> STAKAPTLPASIFRAYDIRGVVGDTLTAETAYWIGRAIGSESLARGEPCVAVGRDGRLSGPELVKQLIQGLVDCGCQVSDVGMVPTPVLYYAANVLEGKSGVMLTGSHNPPDYNGFKIVVAGETLANEQIQALRERIEKNDLASGVGSVEQVDILPRYFKQIRDDIAMAKPMKVVVDCGNGVAGVIAPQLIEALGCSVIPLYCEVDGNFPNHHPDPGKPENLKDLIAKVKAENADLGLAFDGDGDRVGVVTNTGTIIYPDRLLMLFAKDVVSRNPGADIIFDVKCTRRLIALISGYGGRPVMWKTGHSLIKKKMKETGALLA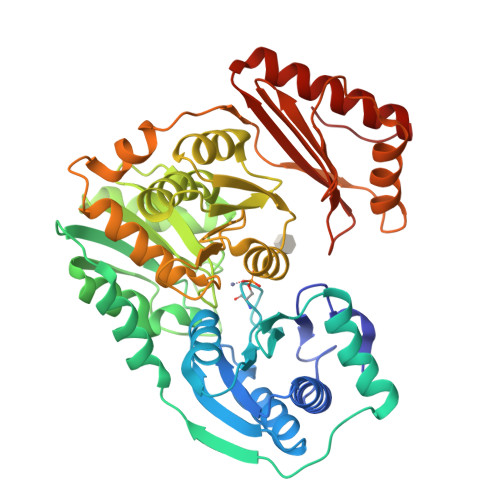GEMSGHVFFKERWFGFDDGIYSAARLLEILSQDQRDSEHVFSAFPSDISTPEINITVTEDSKFAIIEALQRDAQWGEGNITTLDGVRVDYPKGWGLVRASNTTPVLVLRFEADTEEELERIKTVFRNQLKAVDSSLPVPF> RALEVERTVSLAEVYAGLPKDNGPFSLAQEIDKLVSQGSGSAGSGNNNLAFGAGTDTKTSLQASVSFADLKIREDYPASLGKIRRIKQISVTLPALLGPYQDVQAILSYGDKAGLANGCEALAVSHGMNDSGQFQLDFNDGKFLPFEGIAIDQGTLTLSFPNASMPEKGKQATMLKTLN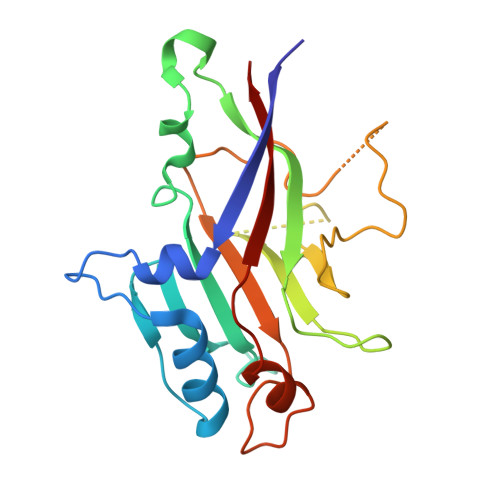DIILHIRYTIK Syntenin is a small intracellular scaffold protein that contains two PSD‐95, Discs‐large, ZO‐1 (PDZ) domains that bind SDC, an N‐terminal domain that binds ALIX (via three LYPxL motifs), and a short C‐terminal domain regulating the conformation of the protein and accessibility of its domains (Baietti et al., 2012; Grootjans et al., 1997; Saito, Nishioka, Iwatsuki, Kumagai, & Sasaki, 1975). The PDZ domains of syntenin bind the C‐termini of the SDCs (Grootjans et al., 1997), but bind also to PIP2 (Zimmermann et al., 2002) and several other membrane proteins, including CD63 (Latysheva et al., 2006). In contrast, SDC‐syntenin‐ALIX binding regulates the formation of endosomal intraluminal vesicles and the secretion of CD63+ exosomes that contain syntenin, C‐terminal fragments of the SDCs (SDC‐CTFs) and potential SDC‐cargo such as ligand‐engaged receptors (Baietti et al., 2012). Since syntenin activity strictly depends on the functionality of its PDZ domains (Baietti et al., 2012; Grootjans et al., 1997; Grootjans, Reekmans, Ceulemans, & David, 2000; Koo et al., 2002; Lambaerts et al., 2012; Luyten et al., 2008; Meerschaert et al., 2007; Zimmermann et al., 2002; Zimmermann et al., 2005; Zimmermann et al., 2001), we aimed to develop syntenin PDZ inhibitors and investigate their potential utility to control cellular phenotypes as well as exosomal‐releases.

Molecular modelling studies, relying on the X‐ray structure of C58 and MOE/Pymol tools, suggested that addition of one carbon spacer in the compound structure could maintain both the canonical binding mode and, the face‐to‐face π‐stacking with Phe213, while slightly increasing the distance between the hydrophobic thioether‐chlorophenyl moiety and the polar protein backbone. Moreover, better torsion angles, closer to optimal geometry (60°), with favourable staggered conformation on the flexible carbohydrate moiety, were also anticipated for this C58 analogue. A new compound with one carbon spacer, further called SyntOFF, was synthesized in three steps from the commercial four‐chlorothiophenol. The small structural modification, consisting in the introduction of a single methylene group as a spacer, resulted in a > 10‐fold improvement of the affinity as compared to C58 (IC50 = 37 µM). SyntOFF reached the reference ligand efficiency (Hopkins, Groom, & Alex, 2004) threshold of 0.30 kcal/mol/atom, starting from the C58 moderate 0.24 kcal/mol/atom value, highlighting the optimal introduction of an additional one carbon spacer in the structure of the C58 (compare Figure 5b and 2b). SyntOFF accordingly inhibited the syntenin‐SDC2 interaction by 96% at 400 µM in HTRF, while the methyl ester intermediate and very close analogue cSyntOFF proved to be inactive. SyntOFF appeared selective for syntenin, not affecting Erbin‐P0071 or GRASP55‐JAM‐B complexes in HTRF. In BIAcore, using DMSO as vehicle, SyntOFF displayed a KD value of 130 µM for syntenin‐PDZ tandem plus C‐terminal domain.

>GAMDPREVILCKDQDGKIGLRLKSIDNGIFVQLVQANSPASLVGLRFGDQVLQINGENCAGWSSDKAHKVLKQAFGEKITMTIRDRPFERTITMHKDSTGHVGFIFKNGKITSIVKDSSAARNGLLTEHNICEINGQNVIGLKDSQIADILSTSGTVVTITIMPAF[4x]> TRSG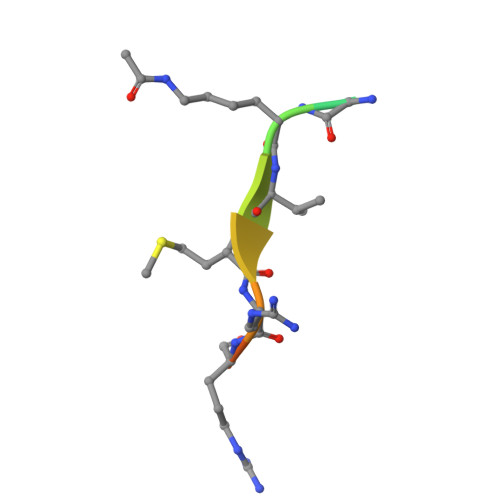KVMRRLRR>GDAAKGEKEFNKCKTCHSIIAPDGTEIVKGAKTGPNLYGVVGRTAGTYPEFKYKDSIVALGASGFAW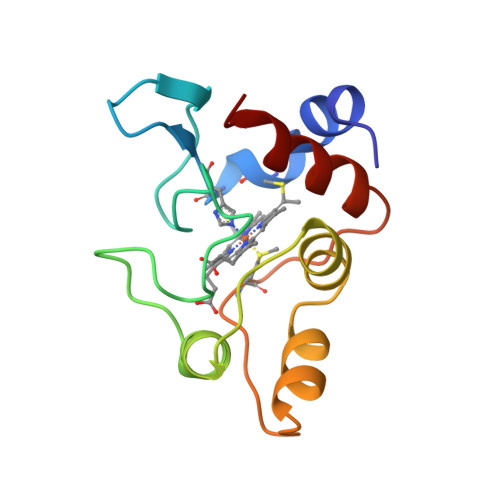TEEDIATYVKDPGAFLKEKLDDKKAKTGMAFKLAKGGEDVAAYLASVVK[2x]> MMNIIKTLFCSMKMVLLLIGIYATACGIATFIEKYEGTLAARLWVYDAFWFEILHIWLVACLIGCFITSKAWQRKKYASLLLHASFIVIIIGAGITRYYGFEGLMNLREGQSVNFISTNTHYIFIQIKNPQGDVESVRIPTYIDEKVNHKINQHLTFFGKPLTLHTEEFTAKQ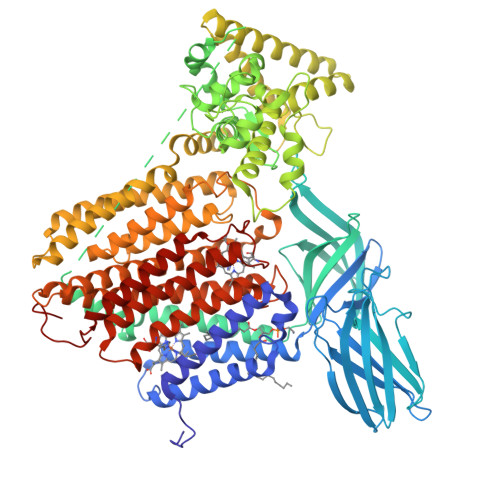VNMSELFILNASIDFLGKNEKTLIMRDGNNAPTKENITMLEIEGYKIFLAWGIDNIALPFSIKLKKFELERYPGSNSPASYTSEVEVLDGQNPPLPFRIFMNNVLDYGGYRFFQSSYHPDEKGSILSVNNDPGKTPTYIGYAMLILGVIWLLFDKNGRFATLGRFLKTQKFFSLMLCSALCYALSSPQIAYASTQSQTDFQPLSENEIPPLQDIPSMIKALADTSSLTNDFDRILVQDFGGRIKPMHTLANEYIHKLTQQRTFKGLNPSQVFLGMLFYPQEWQSIQMIATKSPKLRQILGLDENQKHIAYIDVFTPQGQYILQNYVEAANLKSPSLRDTFEKDVISVDERINYAFLIYTGQVLRIFPDNKSPNNQWLYPLQAISSAVAQDDTKKAKELMQIYKKFAQGMQQGINTHNWQEAAQATRDIRTFQQNNGGSLLISPAKVDSEIWLNLYNPFYQLTYPYIFISIVLFIIVLVGILKNTPTRPLIHKVFYILLFALFILHTCGLGLRWYVSEHAPWSNAYESMLYIAWAAILSGVVFFRRSNLALCASSFLAGMTLFVANLGDMDPQIGNLMPVLKSYWLNIHVSVITASYGFLGLCFMLGLITLIMFLLRNEKRSQVDCSILSLSALNEMSMILGLFLLSVGNFLGGIWANESWGRYWGWDSKETWALISIGVYAIILHLRFVVPKNFPFIFASASVIGFFSVLMTYFGVNYYLTGMHSYAAGEAEPVPLWVELMVAGIILLIIIASRKRVLDMPHLHHHHHH> MMAKNYIARQDGLWTVISLTPDVCKTPVGSSTPPVPYAVIASLGDAVQTVQTVKANGHPVLVLDQSIIPYTKGDEPGVAKGVKSGTVGDICEPLEHSRTVFAGGKPVLRHFDKFWMNARNTTGLIIGQPPVAADSVSKADPAPEPETKEEQSIWDTMLMIQTDQSRAQIEAAPVLLDITIGAAKAFWNQFPDLATILGQGAAMQSAGEMQMNGAMLSAMGMDEMGEAQYRMGEEVMAHAGDFNLDEYRLKMSNRNQEIGGMAYDYGSLVLGGYGLARGGFMGLKTMRTASKLVHEGEAGGKFAAHMMKMDNAEDAATDAEKLADDVVPEGRDGANIKGETQGNGDRGDGVNSMLCTKSGEPVDIGTGDFLQHFSVLSLPGSLPLTLSRFYRSQAKGTGIFGPKWTDEWSCMLTVHGNDMHFTNHEGVDLYYRIPQNGIFRDTANSRQAYYRLSGDIRDELTIFDRRSQHSQIFSLTDNGIYLLSAIHDRYGNRADFIRTEGLLTGIHHSDGYTLALGWQQRQLVSIDLATPQRQRLVTCHYDKNGYLAECDTIQFSHLWHEYTSEGWMTRWRDTDKTCVDIVYDTLGRTVSTLSTEGYFDDQFLYNDDEKCTTYLDAEGGETRYWYNGDGLVTRSIDPLGREETSVWENTRLRSRTDALGRTTAYDYNNEGEISRVSL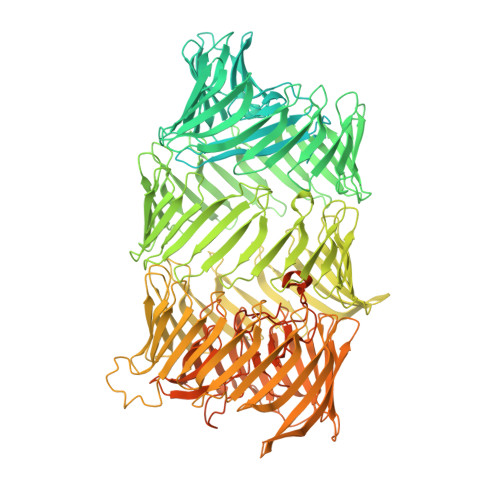PGGYSLYYDYNEHGQLTRLSAPGNQVWLWEYDGKGSMVCLTDPQGRQQQFSYSEHGDLLRQIMPNGATWRWSHDALHQVRATTAPDGGVTQTEQDILGRLLSVKDPLGYTTQFRYSKNHAGPQGSVEEIRRPDGVRELMRQNSEKLPESFTDGEGNTTRYEYGAFDLLTAVIRPDGERLACRYDKLTRLTEITNAEGEHYRLRYDKAGQLVAETDFTGRTLTYSYDAAGRCIRTTFPDGTHLNRQYSTTDQVTREEVAQGDSDRVLSCTTFIYDALSRLTEARNNDATVTYEYDDASRVTAETINGRRTEYNYDPDQDTVSQRTTAGITECFTRGLTGELTQWQIDGHTPLTLEHDLRGQEISRQSEAGFSLRQNYTPTGMLTGQQAGDLTEQNPHYWRNNTLQRQWLYDKAYNLTMISDSLRGTMVNSVTANDQISHATWTGSSDIPMREERFAYDRNLNITRRQTQVNGVPDSEAYQHQQHGRVTSREYKAWRHTTTRINPDSGMPEEGQFVRVIRDEQTTWKYDVNGRLVEKLIDKGGYRPLRWRYRWDARSQLTGLETPEGERREYKYDPFGRRISKRCTNRDRPGTDFHWNGDQLTEEIPVGTDGTPEYENAIRWIYEPGSFTPLARYEKGQLHYTITDTVGRIQELLTEDGTIVWRGKQHLWGREEGRNKDDAPSCRLRFPGQYEDEESGLYYNRFRYYDCEAGQYLCADPIGLRGGINLYAYAPNPLSWIDPLGLKCGETAQPEWTNHRYKHFPPKNKSWKDIIKSTKTGPAKYMHDIDIKTLEYDVFNTGMPATNGKPWKVKNIGKVIGASEGKESQWMRVELSGGTIHGHPISIDEFRRLTTQ> MLCFDSERMNWYYHVLARRPYLVVVSIAVYCVACIIVALVLNKLPDFSDPTLGFETRGTKIGERLTAWYNLLQETDHHGALFSNPSDLWERRRVEQGYVETKLHPNHRRRKNKHKNRNKNKRRKEQNQSSHEHHDVAQKMMQFKKRLKATSSPSPNLGFDTWIGDSGVFRDYEITNDSASSSLEPTRRTEQIEYGHNTTSVDEEEHQQRVQTKKSTWRLLKQAATLPTDGWADMHRRQPIEGFFCDSSPRKEYSHFVVQRIGPNATDSLFDLNGLLAMCQLQDQITEVPSYRAFCEPEMLTTECCRPWSLPNYAAMLANKSSCFDLTTEDVTSLHTLLLGCYEYFHDLKMDNHCNEIPHCRAPEECKRLNIVFNVLNFLTDFSFIKSNDSNVYLKYAMIFIPVAQSNRLLPLFHEWEDVELINELVEVVAMDLGLENELFNELLLTDVWLVSLGGTFVMASVWLYTGSAFITLMSCVAICFSLGLAYFFYAIVLEFEFFPYMNLLAVVVIIGIGADDVFLFLKIWHCVLTERFSNRCTLTTQSQSALPTLENSDHTESLENIMALTMRHAAASMFVTSLTTAGAFYASYSSSITAIKCFGIFAGTVVVTNYLLMITWLPASVSIMERLFATRMSCHHPMSIKLIHACKKSINRFCQMFEECITKSIMNYAYLWLLIFGALGASSAVIVFWYPGLQLPEKSHFQLFVSKHPFEVYSSLKQQFWFEKPLQAYYNFKMHMHFVWGVQAVDDGDYTNPNSYGHLHYDNNFNVSSRPAQLWILDFCQSVRQQPFYKETLGMLLPNCFIENLIDYMKRRCIDDMDSTRKDRSPCCDAQFPFEPHIFEYCLPQSISNMYDTTFFRPGVAGPKFAEAPRLETEDYLGMSGNESAEYSTNGSFTPLLVKALVIEFESNVAYSTIYANIRQFYESVEHWFQMQLKTAPPELQGGWFTSDLKFYNVQDTLSHDTFVAICLAMAASLAVLLCFTVNILISIYAVLTVSLSIFNTVAVLILLGWQLNILESIAVSTAIGLAVDFSLHYGIHYRMSPVKERLAATQFVLSRIIGPTVMAATTTGLAGGIMMASNILPYIQIGVFLVVVMIVSWFYATFFLMSLLRVAGPQHGFLELKWPLWSKRSSGSSKFYERKPSQVIASEQLLTPTSSAIVELANSETHELESLNSNSLIKTISGIESAHALSSLPRDFEHSFQTMHECKYQTYPSTSN;> MDNHSSVPWASAASVTCLSLDAKCHSSSSSSSSKSAASSISAIPQEETQTMRHIAHTQRCLSRLTSLVALLLIVLPMVFSPAHSCGPGRGLGRHRARNLYPLVLKQTIPNLSEYTNSASGPLEGVIRRDSPKFKDLVPNYNRDILFRDEEGTGADRLM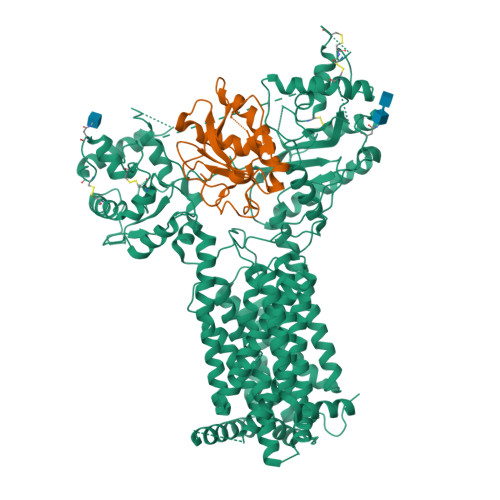SKRCKEKLNVLAYSVMNEWPGIRLLVTESWDEDYHHGQESLHYEGRAVTIATSDRDQSKYGMLARLAVEAGFDWVSYVSRRHIYCSVKSDSSISSHVHGCFTPESTALLESGVRKPLGELSIGDRVLSMTANGQAVYSEVILFMDRNLEQMQNFVQLHTDGGAVLTVTPAHLVSVWQPESQKLTFVFADRIEEKNQVLVRDVETGELRPQRVVKVGSVRSKGVVAPLTREGTIVVNSVAASCYAVINSQSLAHWGLAPMRLLSTLEAWLPAKEQLHSSPKVVSSAQQQNGIHWYANALYKVKDYVLPQSWRHD>[6x]MSRVS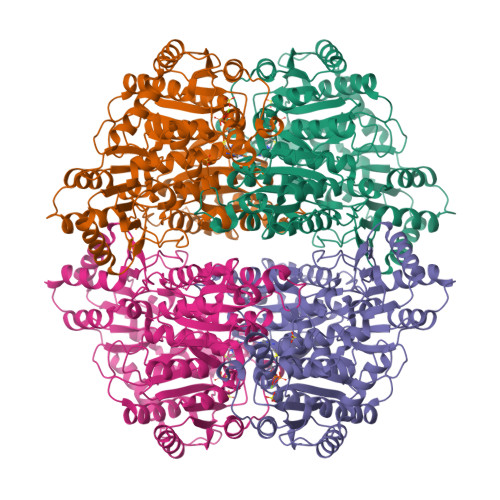TAPSGKPTAAHALLSRLRDHGVGKVFGVVGREAASILFDEVEGIDFVLTRHEFTAGVAADVLARITGRPQACWATLGPGMTNLSTGIATSVLDRSPVIALAAQSESHDIFPNDTHQCLDSVAIVAPMSKYAVELQRPHEITDLVDSAVNAAMTEPVGPSFISLPVDLLGSSEGIDTTVPNPPANTPAKPVGVVADGWQKAADQAAALLAEAKHPVLVVGAAAIRSGAVPAIRALAERLNIPVITTYIAKGVLPVGHELNYGAVTGYMDGILNFPALQTMFAPVDLVLTVGYDYAEDLRPSMWQKGIEKKTVRISPTVNPIPRVYRPDVDVVTDVLAFVEHFETATASFGAKQRHDIEPLRARIAEFLADPETYEDGMRVHQVIDSMNTVMEEAAEPGEGTIVSDIGFFRHYGVLFARADQPFGFLTSAGCSSFGYGIPAAIGAQMARPDQPTFLIAGDGGFHSNSSDLETIARLNLPIVTVVVNNDTNGLIELYQNIGHHRSHDPAVKFGGVDFVALAEANGVDATRATNREELLAALRKGAELGRPFLIEVPVNYDFQPGGFGALSI> MAEVLVVTS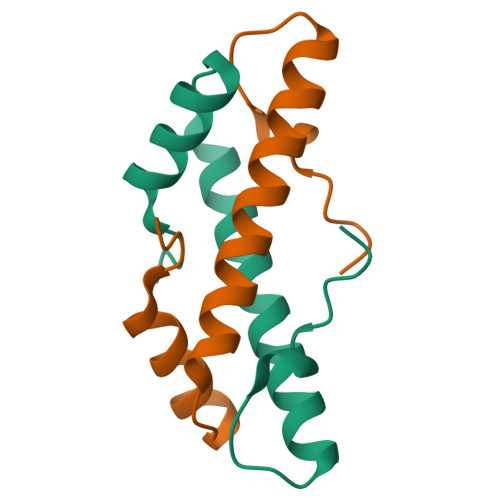KVKKLIKEKGQMNTSAETIDVLSKAIEQLCLKGVESAKADGRKTVMARDIVIDHL>[2x]MTKRVAVIGAGPSGLAQLRAFQSAADQGAEIPEIVCFEKQANWGGLWNYTWRTGLDENGEPVHCSMYRYLWSNGPKEGLEFADYSFEEHFGKQIASYPPRAVLFDYIEGRVHKADVRKWIRFNSPVRWVSYDAETAKFTVTAHNHETDSTYSEDFDHVICASGHFSTPNVPFYEGFDTFNGRIVHAHDFRDARE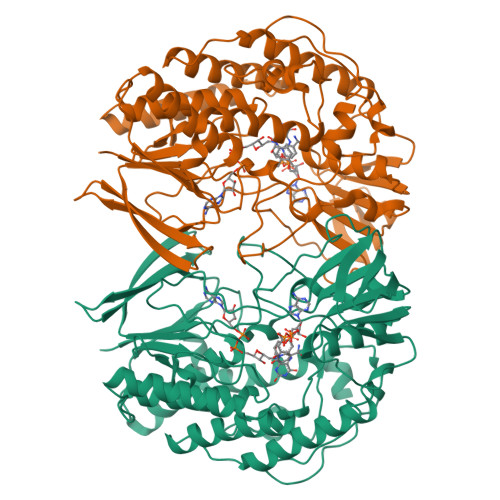FEGKDVLVMGASSSAEDIGSQCWKYGAKSITSCYRSAPMGYAWPDNWEEKPALEKLTGKTAHFADGSTRDVDAIILCTGYKHFFSFLPDDLRLKTANRLATADLYKGVAYVHNPAMFYLGMQDQWFTFNMFDAQAWWVRDAILGRITLPKDKAAMLADVAERETREEASDDVKYAIRYQADYVKELVAETDYPSFDIDGACDAFFEWKKHKAKDIMAFRDNSYKSVITGTMAPVHHTPWKEALDDSMEAYLQNHHHHHH>MSLSTARIMLV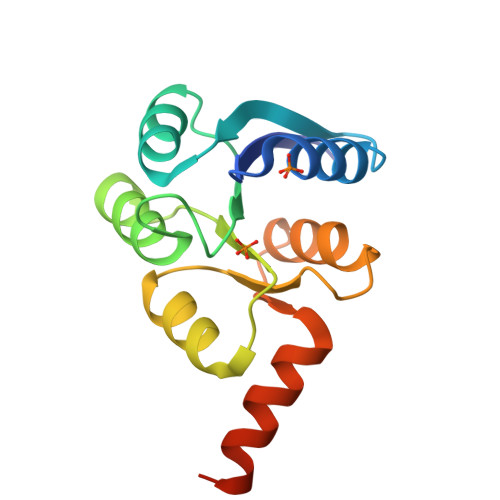DDHPIVREGYRRLIERRPGYAVVAEAADAGEAYRLYRETTPDIVVMDLTLPGPGGIEATRHIRQWDGAARILIFTMHQGSAFALKAFEAGASGYVTKSSDPAELVQAIEAILAGRRAMSPDIAQEIAEERVEGREGHHHHHH[4x]>GSTSMSATRRIVLGLIPADGIGKEVVPAARRLMENLPAKHKLKFDFIDLDAGWGTFERTGKALPERTVERLKTECNAALFGAVQSPTHKVA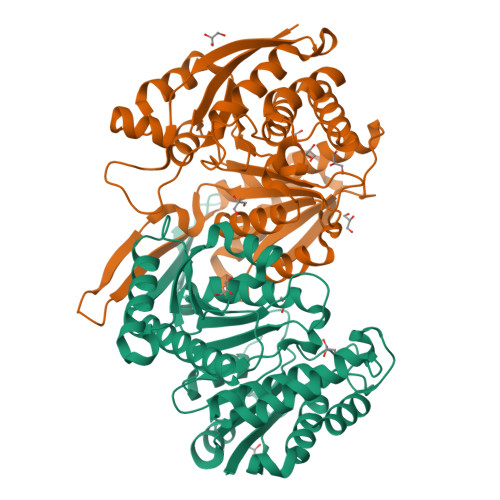GYSSPIVALRKKMGLYANVRPVKSLDGAKGKPVDLVIVRENTECLYVKEERMVQNTPGKRVAEAIRRISEEASTKIGKMAFEIAKSRQKIRESGTYSIHKKPLVTIIHKSNVMSVTDGLFRESCRHAQSLDPSYASINVDEQIVDSMVYRLFREPECFDVVVAPNLYGDILSDGAASLIGSLGLVPSANVGDNFVMSEPVHGSAPDIAGRGIANPVATFRSVALMLEFMGHQDAAADIYTAVDKVLTEGKVLTPDLGGKSGTNEITDAVLANIHN[2x]>[2x]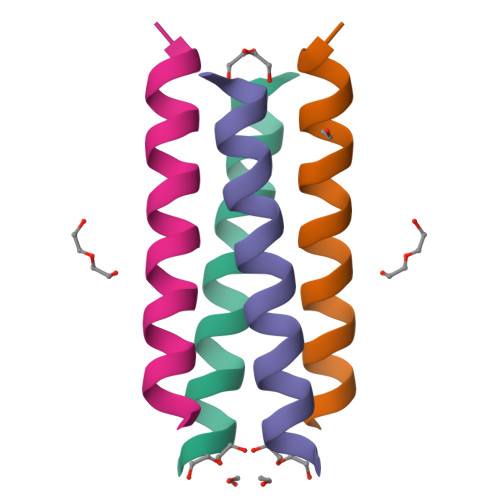GNADEXYKEXEDXQERLRKLRKKLRSG> ISDPVELLKRAEKKGVPSSGFMKLFSGSDSYKFEEAADLCVQAATIYRLRKELNLAGDSFLKAADYQKKAGNEDEAGNTYVEAYKCFKSGGNSVNAVDSLENAIQIFTHRGQFRRGA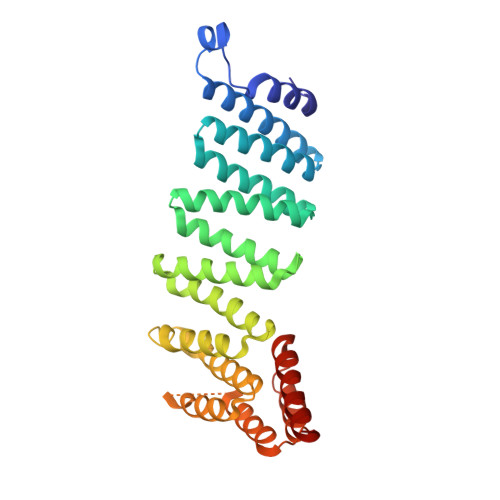NFKFELGEILENDLHDYAKAIDCYELAGEWYAQDQSVALSNKCFIKCADLKALDGQYIEASDIYSKLIKSSMGNRLSQWSLKDYFLKKGLCQLAATDAVAAARTLQEGQSEDPNFADSRESNFLKSLIDAVNEGDSEQLSEHCKEFDNFMRLDKWKITILNKIKESIQQQEDDLL>[2x]MAHHHHHHMSKKRVLTGVTTTGTPHLGNYVGAIRPAVRAAQNPDTESFLFLADYHGIIKCHEQEMIHQ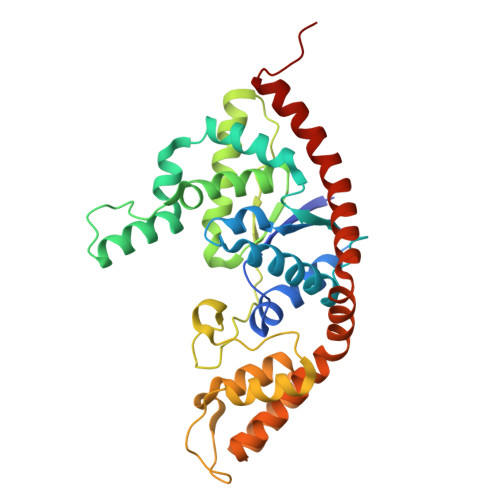STQAVAATWLACGLDPERTTFYRQSDIPEVMELNWILTCITAKGLMNRAHAYKAAVQANAENGQEDPDFGVEMGLFSYPILMTADILMFNANEVPVGRDQIQHVEMARDIAGRFNHRFQELFTLPEVKIDENVELLVGLDGRKMSKSYGNTIPLWENDKKTQKSVNKIITNMKEPGEPKQPDESPLFEIYKAFSTPSETAEFTQMLADGLAWGEAKKLSAAKINAELAELRERYNALTSNPSQIEEILQAGAQKARKEARELLDKVRDAVGIRPLK N-({3-[4-(5-amino-1H-pyrrolo[3,2-b]pyridin-2-yl)-5-hydroxy-1H-pyrazol-1-yl]phenyl}methyl)-N'-phenylurea 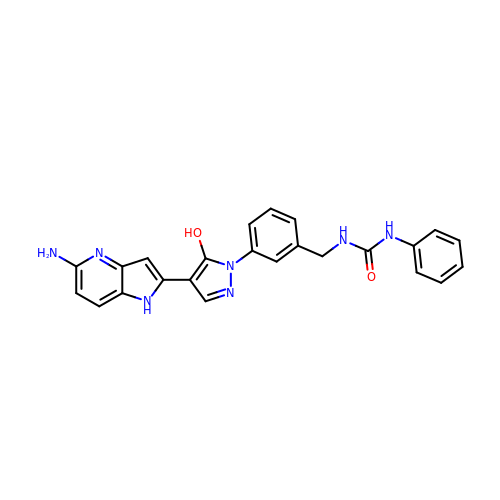| C24 H21 N7 O2 | UTXKUUYFKOVOOK-UHFFFAOYSA-N>DYKDDDDKDYKDDDDKDYKDDDDKHHHHHHENLYFQGVSRMGWGGRRRRLGRWGDLGPGSVPLLPMPLPPPPPPSCRGPGGGRISIFSLSPAPHTRSSPSSFSPPTAGPPCSVLQGTGASQSCHSALPIPATPPTQAQPAMTPASASPSWGSHSTPPLAPATPTPSQQCPQDSPGLRVGPLIPEQDYERLEDCDPEGSQDSPIHGEEQQPLLHVPEGLRGSWHHIQNLDSFFTKIYSYHQRNGFACILLEDVFQLGQFIFIVTFTTFLLRCVDYNVLFANQPSNHTRPGPFHSKVTLSDAILPSAQCAERIRSSPLLVLLLVLAAGFWLVQLLRSVCNLFSYWDIQVFYREALHIPPEELSSVPWAEVQSRLLALQRSGGLCVQPRPLTELDIHHRILRYTNYQVALANKGLLPARCPLPWGGSAAFLSRGLALNVDLLLFRGPFSLFRGGWELPHAYKRSDQRGALAARWGRTVLLLAALNLALSPLVLAWQVLHVFYSHVELLRREPGALGARGWSRLARLQLRHFNELPHELRARLARAYRPAAAFLRTAAPPAPLRTLLARQLVFFAGALFAALLVLTVYDEDVLAVEHVLTAMTALGVTATVARSFIPEEQCQGRAPQLLLQTALAHMHYLPEEPGPGGRDRAYRQMAQLLQYRAVSLLEELLSPLLTPLFLLFWFRPRALEIIDFFHHFTVDVAGVGDICSFALMDVKRHGHPQWLSAGQTEASLSQRAEDGKTELSLMRFSLAHPLWRPPGHSSKFLGHLWGRVQQDAAAWGATSARGPSTPGVLSNCTSPLPEAFLANLFVHPLLPPRDLSPTAPCPAAATASLLASISRIAQDPSSVSPGGTGGQKLAQLPELASAEMSLHVIYLHQLHQQQQQQEPWGEAAASILSRPCSSPSQPPSPDEEKPSWSSDGSSPASSPRQQWGTQKARNLFPGGFQVTTDTQKEPDRASCTD[3x]

Macroautophagy/autophagy is a fundamental aspect of eukaryotic biology, and the autophagy-related protein ATG9A is part of the core machinery facilitating this process. In addition to ATG9A vertebrates encode ATG9B, a poorly characterized paralog expressed in a subset of tissues. Herein, we characterize the structure of human ATG9B revealing the conserved homotrimeric quaternary structure and explore the conformational dynamics of the protein. Consistent with the experimental structure and computational chemistry, we establish that ATG9B is a functional lipid scramblase.

Full-length ATG9B, N-terminally tagged with a triple FLAG epitope, was transiently overexpressed in Expi293 cells. The protein was extracted from membranes into detergent micelles and affinity purified using anti-FLAG resin. Further image processing with and without C3 symmetry imposed resulted in 3D reconstructions of ATG9B homotrimer at a global resolution of 4.2 Å (EMD-17789) and 4.6 Å (EMD-17790), respectively, while the local resolution in the core regions of the symmetry-imposed structure ranged between 3.2 and 3.8 Å. Although imposing C3 symmetry during refinement improved overall resolution, it introduced minor artifacts in the cryo-EM map that were absent when the volume was refined without symmetry. Most of the backbone and side chains of residues corresponding to ATG9B amino acid positions 191–674 were visible in the cryo-EM maps. By contrast, the N- and C-terminal regions were not, presumably due to conformational variability and/or intrinsic disorder. ATG9B forms a homotrimer with a pore at its center connected to perpendicular branches formed at the protomer interfaces. Each protomer has a lateral branch that connects to the central pore and the perpendicular branches. As reported for other ATG9 domain proteins, the ATG9B subunits share an extensive interaction interface within the homotrimer, with an approximately 2,494Å2 buried molecular surface area per subunit. The conformation of our consensus structure is in a transition state between the open (state A) and closed (state B) conformers reported for ATG9A.>MAAPQLFRALVSAQWVAEALKAPRSSQPLKLLDASWYLPKLGRDARREFEERHIPGAAFFDIDRSSDHTSPYDHMLPNATHFADYAGSLGVSAATHVVIYDGSDQGLYSAPRVWWMFRAFGHHSVSLLDGGFRHWLNQNLPISSGKSHSEPAEFSAQLDPSFIKTHEDILENLDARRFQVVDARAAGRFQGTQPEPRDGIEPGHIPGSVNIPFTEF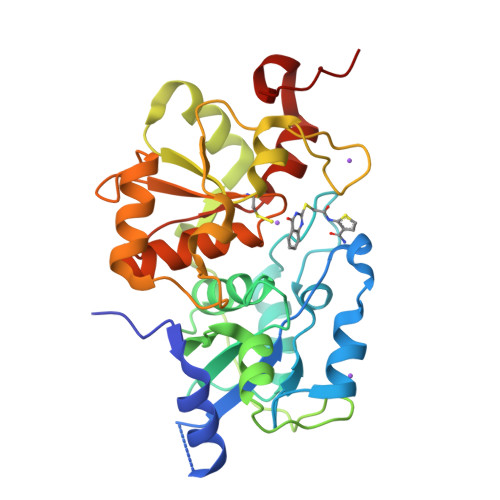LTNEGLEKSPEEIKRLFKEKKVDLSKPLVATCGSGVTASHVVLGAFLSGKSDVPVYDGSWVEWYMRAQPEHIISEGRGKTQ[2x]> GSRG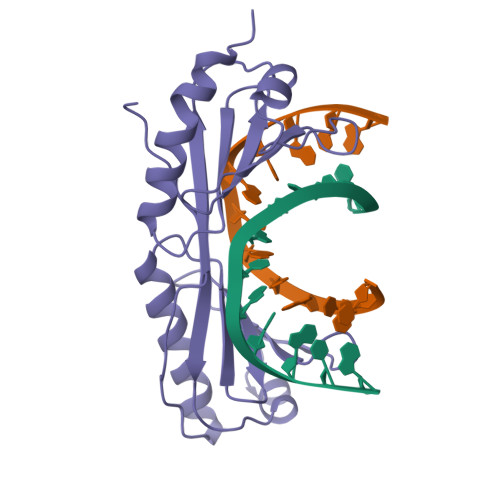SGIVPQLQNIVSTVNLGCKLDLKTIALRARNAEYNPKRFAAVIMRIREPRTTALIFSSGKMVCTGAKSEEQSRLAARKYARVVQKLGFPAKFLDFKIQNMVGSCDVKFPIRLEGLVLTHQQFSSYEPELFPGLIYRMIKPRIVLLIFVSGKVVLTGAKVRAEIYEAFENIYPILKGFRKTT>[2x]AMDLRVGRKFRIGRKIGSGSFGDIYHGTNLISGEEVAIRLESIRSRHPQLDYESRVYRYLSGGVGIPFIRWFGREGEYNAMVIDLLGPSLEDLFNYCHRRFSFKTVIMLALQMFCRIQYIHGRSFIHRDIKPDNFLMGVGRRGSTVHVIDFGLSKKYRDFNTHRHIPYRENKSLTGTARYASVNTHLGIEQSRR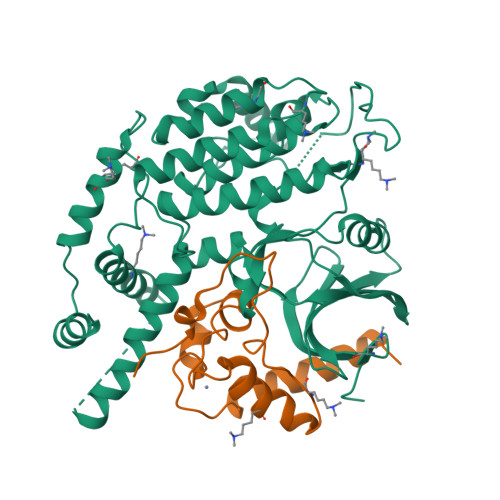DDLESLGYVLIYFCKGSLPWQGLKATTKKQKYDRIMEKKLNVSVETLCSGLPLEFQEYMAYCKNLKFDEKPDYLFLARLFKDLSIKLEYHNDHLFDWTMLRYTKAMVEKQRDLLIEKGDLNANSNAASASNSTDNKSETFNKIKLLAMKKFPTHFHYYKNEDKHNPSPEEIKQQTILNNNAASSLPEELLNALDKGMENLR;>EATECLTRSNLKKLQEKIFDRELNDIACDHCLCSTENRRDIKYSRLWFLFELEMSENWNENLRLSCYNKYVYSAIDESWKMENILLKEQEKHYEYFPIGQLLIPN[2x]> MSAPRAEEQPSRSGERQPLVARGPRGPRRWRRTAAAAVLLVQMLERAAFFGVTSNLVLYLNSLNFNWDGQQASRATLLFLGASYLLAPVGGWLADVYLGRFLTISLSLLLYLAASGLLLTTITNDGRRSFCGEMPELPLEPACPSSSCQGSWSSPYCATTLYLVLLLLALAASSVRSTLTSFGADQVMDLGRDATRRFFNWFYWSINLGAILSLLVVAFIEQNISFLWGYSIIVGLVGLAFFIFLFATPVFITKPPTGSQVSSMLKLAFQNCCPCRRSSSRDSESAHLLPDQRSNQPGPSPQEDMANFQVLVKILPVMVTLVPYWMVYFQMQSTYVLQGLHLHIPNIFRTNPNISLLLRSDSSNYRIPEAWLLLANVAVILILIPVKDHLIDPLLLRCKLLPSSLQKMALGMFFGFTSIIVAGVLEKERLQYIAANQTVPQLIGKDLYYAAPLSIWWQIPQYLLIGVSEIFASIPGLEFAYSEAPRSMQGAIMGIFFCLSGVGSLLGSGLVALLSFPGGWMYCPKDFGNINNCQMDRYFFLLAGIEAVTAVLFLWIA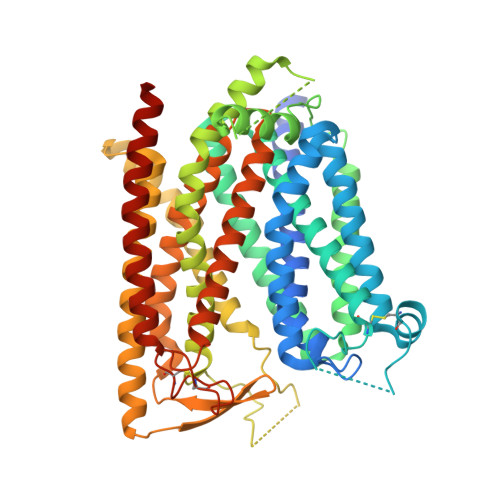GRYERTRQDPASQRSSSRVRG> HHAADYVLYKDATKPVEDRVADLLGRMTLAEKIGQMTQIERLVATPDVLRDNFIGSLLSGGGSVPRKGATAKEWQDMVDGFQKACMSTRLGIPMIYGIDAVHGQNNVYGATIFPHNVGLGATRDPYLVKRIGEATALEVRATGIQYAFAPCIAVCRDPRWGRCYESYSEDRRIVQSMTELIPGLQGDVPKDFTSGMPFVAGKNKVAACAKHFVGDGGTVDGINENNTIINREGLMNIHMPAYKNAMDKGVSTVMISYSSWNGVKMHANQDLVTGYLKDTLKFKGFVISDAEGIDRITTPAGSDYSYSVKASILAGLDMIMVPNKYQQFISILTGHVNGGVIPMSRIDDAVTRILRVKFTMGLFENPYADPAMAEQLGKQEHRDLAREAARKSLVLLKNGKTSTDAPLLPLPKKAPKILVAGSHADNLGYQCGGWTIEWQGDTGRTTVGTTILEAVKAAVDPSTVVVFAENPDAEFVKSGGFSYAIVAVGEHPYTETKGDNLNLTIPEPGLSTVQAVCGGVRCATVLISGRPVVVQPLLAASDALVAAWLPGSEGQGVTDALFGDFGFTGRLPRTWFKSVDQLPMNVGDAHYDPLFRLGYGLTTNATKKY

In the barley β-d-glucan glucohydrolase, a glycoside hydrolase family 3 (GH3) enzyme, the Trp286/Trp434 clamp ensures β-d-glucosides binding, which is fundamental for substrate hydrolysis during plant growth and development. HvExoI folds into a two-domain structure consisting of an (α/β)8 barrel (domain 1) and an (α/β)6 sandwich (domain 2) with a 13 Å-deep active site pocket embracing the subsites −1 and +1, positioned at the interface between the two domains. HvExoI catalyses the hydrolytic removal of nonreducing glucose (Glc) moiety from a broad spectrum of poly- and oligomeric β-d-glucosides. The crucial role of substrate binding in HvExoI implies a pair of the aromatic Trp286 and Trp434 residues that form a clamp at the +1 subsite, which is positioned next to a pocket-shaped site at the −1 subsite, housing the Asp285 and Glu491 catalysts.

G6SG-OMe bound tightly to native and WT recombinant HvExoI with the respective Ki values of 0.1 ×10−3 M and 0.2 ×10−3 M, hinting that this thio-analogue should be observed in the active sites of WT and mutants. This is what we indeed observed in WT, and the W286A, W286Y, W286F, W434A, W434F, W434H, and W434Y mutants, where well-defined electron density maps of G6SG-OMe and tight H-bond networks that were formed through eight to ten residues (Asp95, Lys206, His207, Arg158, Tyr253, Asp285, Arg291, Glu491, Trp286, and Trp434). We noted that the quality of the G6SG-OMe electron density map slightly declined in W286Y but that these maps were well-formed in W286A and W286F, suggesting that in the W286Y mutant the process of ligand-binding in (or near) the active site may have been perturbed. While the Glc moieties of G6SG at the −1 subsite were oriented nearly identically in WT and mutant structures, the position of the Glc moiety at the +1 subsite varied – it was identical in WT and W286A, while in W434A it was rotated by 120° through the x-axis. Our findings suggest that although the mutations of Trp286 to Ala and His led to folded but inactive enzymes, enzyme activity retention is more sensitive to alterations of Trp286 than Trp434, likely due to the proximity of Trp286 to Asp285, the catalytic nucleophile.5'-O-(N-(L-SERYL)-SULFAMOYL)ADENOSINE | C13 H19 N7 O8 S | 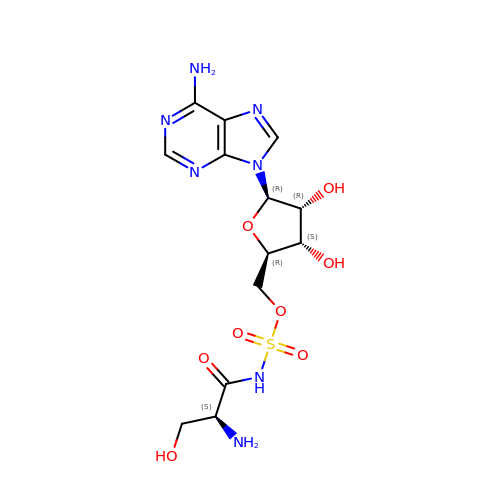HQXFJGONGJPTLZ-YTMOPEAISA-N> GMADEATRRVVSEIPVLKTNAGPRDRELWVQRLKEEYQSLIRYVENNKNADNDWFRLESNKEGTRWFGKCWYIHDLLKYEFDIEFDIPITYPTTAPEIAVPELDGKTAKMARGGKICLTDHAKPLWARNVPKFGLAHLMALGLGPWLAVEIPDLIQKGVIQHKEKCNQ

Analogous to ubiquitination, ufmylation is carried out by a three-enzyme cascade involving E1, E2, and E3 proteins. The E1 UBA5 has three distinct regions: (1) an adenylation domain that binds ATP and magnesium ions; (2) a UFM1-interacting sequence (UIS) spanning amino acids 334 to 346 that holds UFM1 in a trans binding mechanism; and (3) a UFC1-binding sequence (UBS) from 392 to 404 that binds UFC117–21. The adenylated UFM1 is then subjected to a nucleophilic attack by the catalytic C250 of UBA5 to form a thioester bond with the C-terminal glycine of UFM1. This is followed by a trans thiolation process, whereby the UFM1 is transferred to the E2 UFC1 forming a thioester bond with C116 of UFC1. However, UBA5 does not harbor such a domain but instead has a short sequence called UBS that is responsible for the interaction with UFC128.

To further understand how the UFC1 double mutant (Y110A and F121A) affects UFM1 transfer to UFC1, we determined its crystal structure to 2.2 Å resolution. As expected, the double mutant kept the overall UBC fold as observed in WT UFC1 with an RMSD of 0.3 Å2. The main differences were concentrated in the loop harboring the active site Cys. Specifically, Leu 117 Cα moves 1.7 Å away from its position in the WT, and its side chain points towards the position of the missing phenylalanine (F121A). This movement is not feasible in the WT due to steric clashes with F121. Then, to understand how these conformational changes affect UFM1 transfer, we examined our model suggesting that UBA5 Y372 utilizes a cavity on the UFC1 surface. To that end, we measured the volume of this cavity in UFC1 WT and double mutant using CASTp40. While in WT this cavity has a volume of 377 Å3, in the double mutant it becomes 126 Å3. This change probably hampers the ability of UBA5 Y372 to occupy this pocket and therefore affects the recruitment of UBA5 linker to the active site Cys. Taken together, our results suggest that changes in the cavity volume of UFC1 due to the double mutant interferes with the ability of UBA5 to execute its role in desolvation, and accordingly, increasing the pH helps to overcome the defect in transfer.>[4x]MDKEEVKREMKEQEGNPEVKSKR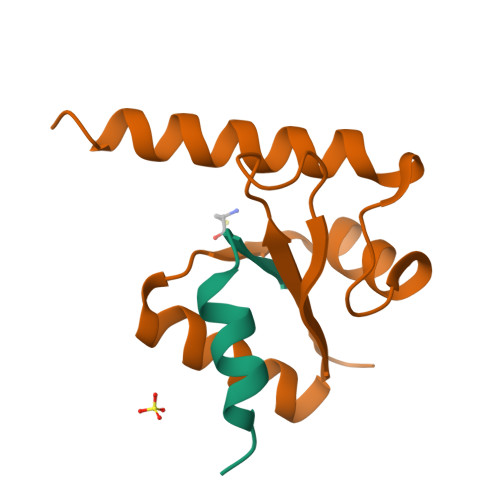REVHMEILSEQVKSDIENSRLIVAN;>PTHITIGIYFKPELMPIPMISVYETNQRALAVRAYAEKVGVPVIVDIKLARSLFKTHRRYDLVSLEEIDEVLRLLVWLEEVENAGKDVIQPQENEVRH[4x]> SPEQAMRERSELARKGIARAKSVVALAYAGGVLFVAENPSRSLQKISELYDRVGFAAAG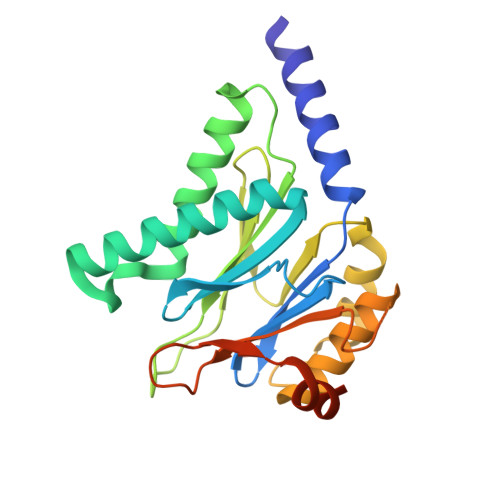KFNEFDNLRRGGIQFADTRGYAYDRRDVTGRQLANVYAQTLGTIFTEQAKPYEVELCVAEVAHYGETKRPELYRITYDGSIADEPHFVVMGGTTEPIANALKESYAENASLTDALRIAVAALRAGSADTSGGDQPTLGVASLEVAVLDANRPRRAFRRITGSALQALLVDQESPQSDGESSG> MARPFKFPRSYAALLADWPVVVLGMCTLLIVVCALVGVLVPELPDFSDPLLGFEPRGTTIGQRLVTWNNMMRNTGYKATLANYPYKYAEEQARSHRDDRWSDDHHERERREVDWNFQKDSFFCDVPSDGYSRVVFASAGGETLWNLPAIKSMCDVDNSRIRSHPQFSDLCQRTTAVSCCPSWTLGNYIAILNNRSSCQKIVERDVSHTLKLLRTCAKHYQNGTLGPDCWDKAARRKDQLKCTNVPRKCTKYNAVYQILHYLVDKDFMTPKTADYAVPALKYSMLFSPTEKGESMMNIYLDNFENWNSSDGITTVTGIEFGIKHSLFQDYLLMDTVYPAIAIAIVLLIMCVYTKSMFITLMTMFAIISSLIVSYFLYRVVFNFEFFPFMNLTALIILVGIGADDAFVLCDVWNYTKFDKPRAETSEAVSVTLQHAALSMFVTSFTTAAAFYANYVSNITAIRCFGVYAGTAILVNYVLMVTWLPAVIVLHERYLLNIFTCFRKPQPQAYDKSCWAVLCQKCRRVLFAVSEASRIFFEKVLPCIVIKFRYLWLIWFLALTVGGAYIVCVNPKMKLPSLELSEFQVFRSSHPFERYDAEFKKLFMFERVHHGEELHMPITVIWGVSPEDSGDPLNPKSKGELTLDSTFNIASPASQAWILHFCQKLRNQTFFHQTEQQDFTSCFIETFKQWMENQDCDEPALYPCCSHCSFPYKQEVFELCIKKAIMELDRSTGYHLNNKTPGPRFDINDTIRAVVLEFQSTFLFTLAYEKMQQFYKEVDSWISHELSSAPEGLSRGWFVSNLEFYDLQDSLSDGTLIAMGLSVAVAFSVMLLTTWNIIISLYAIVSIAGTIFVTVGSLVLLGWELNVLESVTISVAVGLSVDFAVHYGVAYRLAPDPDREGKVIFSLSRMGSAIAMAALTTFVAGAMMMPSTVLAYTQLGTFMMLVMCVSWAFATFFFQCLCRCLGPQGTCGQIPFPTKLQCSPFSHTLSARPGDRGPSKTHAASAYSVDARGQKSQLEHEFYELQPLASHSCTSSEKTTYEEPHTCSEFFNGQAKNLRMPVPAAYSSELTKSPSSEPGSALLQSCLEQDTVCHFSLNPRCNCRDAYTHLQYGLPEIHCQQMGDSLCHKCASTAGGFVQIQSSVAPLKASHQAAEGLLHPAQHMLPPGMQNSRPRNFFLHSVQHFQAQENLGRTSTHST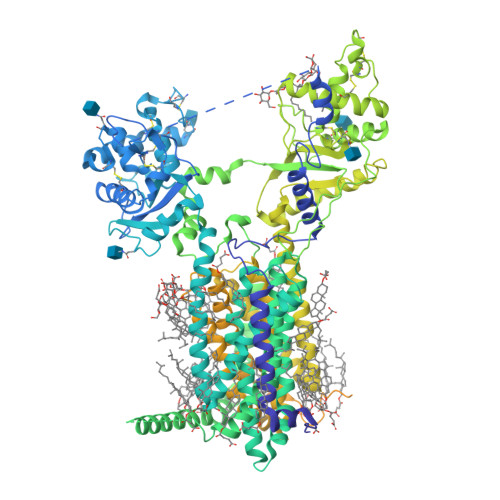DERLPRTAELSPPPSDSRSTESFQRACCHPENNQRRLCKSRDPGDTEGSGGTKSKVSGLPNQTDKEEKQVEPSLLQTDETVNSEHLNHNESNFTFSHLPGEAGCRSCPNSPQSCRSIMRSKCGTEDCQTPNLEANVPAVPTHSDLSGESLLIKTL The zinc-dependent metalloprotease meprin α is predominantly expressed in the brush border membrane of proximal tubules in the kidney and enterocytes in the small intestine and colon. In normal tissue homeostasis meprin α performs key roles in inflammation, immunity, and extracellular matrix remodelling. In contrast to meprin β, meprin α is secreted into the extracellular space, whereupon it oligomerises to form giant assemblies and is the largest extracellular protease identified to date (~6 MDa). Here, using cryo-electron microscopy, we determine the high-resolution structure of the zymogen and mature form of meprin α, as well as the structure of the active form in complex with a prototype small molecule inhibitor and human fetuin-B. Our data reveal that meprin α forms a giant, flexible, left-handed helical assembly of roughly 22 nm in diameter.

Activation of the zymogen was accomplished by way of magnetic trypsin beads. These enabled the cleavage of the pro-peptide and facilitated subsequent removal of trypsin without further dilution of the protein sample by additional purification steps. Comparison between the cryo-EM reconstructions of the latent and activated states reveal subtle conformational changes about the M12A catalytic domain. Accordingly, the steric occlusion of the active site represents the major autoinhibitory mechanism. Upon activation, the two lobes of the M12A catalytic domain collapse around the active site (RMSD 3.3 Å), permitting the formation of a more tightly folded active site core. Upon proteolytic cleavage of the pro-peptide the active is exposed and the M12A protease domain undergoes a conformational relaxation. The exposed active site defines a deep pocket that positions the catalytic glutamic acid in close proximity to the substrate peptide as described for meprin β56. The subunit is a compact triad comprising the globular M12A protease, MAM and MATH domains. The meprin α M12A domain is typical, containing the catalytic zinc ion within the active site. For all variants, the zymogen form was roughly 6 kDa higher in mass than the activated counterpart consistent with the removal of the propeptide.

> WSHPQFEKVPIKYLPEENVHDADFGEQKDISEINLAAGLDLFQGDILLQKSRNGLRDPNTRWTFPIPYILADNLGLNAKGAILYAFEMFRLKSCVDFKPYEGESSYIIFQQFDGCWSEVGDQHVGQNISIGQGCAYKAIIEHEILHALGFYHEQSRTDRDDYVNIWWDQILSGYQHNFDTYDDSLITDLNTPYDYESLMHYQPFSFNKNASVPTITAKIPEFNSIIGQRLDFSAIDLERLNRMYNCTTTHTLLDHCTFEKANICGMIQGTRDDTDWAHQDSAQAGEVDHTLLGQCTGAGYFMQFSTSSGSAEEAALLESRILYPKRKQQCLQFFYKMTGSPSDRLVVWVRRDDSTGNVRKLVKVQTFQGDDDHNWKIAHVVLKEEQKFRYLFQGTKGDPQNSTGGIYLDDITLTETPCPTGVWTVRNFSQVLENTSKGDKLQSPRFYNSEGYGFGVTLYPNSRESSGYLRLAFHVCSGENDAILEWPVENRQVIITILDQEPDVRNRMSSSMVFTTSKSHTSPAINDTVIWDRPSRVGTYHTDCNCFRSIDLGWSGFISHQMLKRRSFLKNDDLIIFVDFEDITHLS> SPTVEECGYSDRVRSITLGNSTITTQECANVVVGYGVWPDYLKDSEATAEDQPTQPDVATCRFYTLDSVQWQKTSPGWWWKLPDALSNLGLFGQNMQYHYLGRTGYTVHVQCNASKFHQGCLLVVCV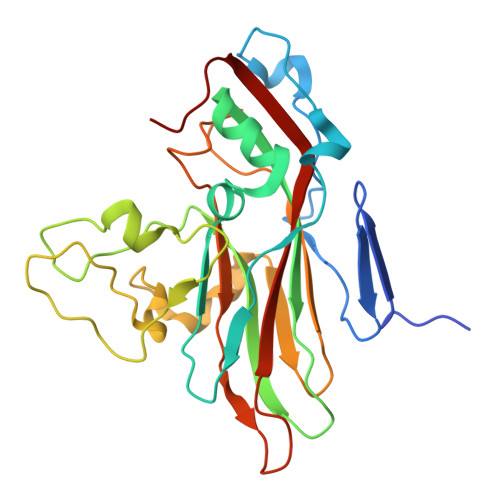PEAEMGCATLDNTPSSVELLGGDSAKEFADKPVASGSNKLVQRVVYNAGMGVGVGNLTIFPHQWINLRTNNSATIVMPYTNSVPMDNMFRHNNVTLMVIPFVPLDYCPGSTTYVPITVTIAPMCAEYNGLRLAGHQ> EQCSAIVPCPGGRCCSQWGYCGNTPAYCCTGCQSNCEETVCGDCPPNSGSAGDGGENGKIISRDMFDELLKRRNDLD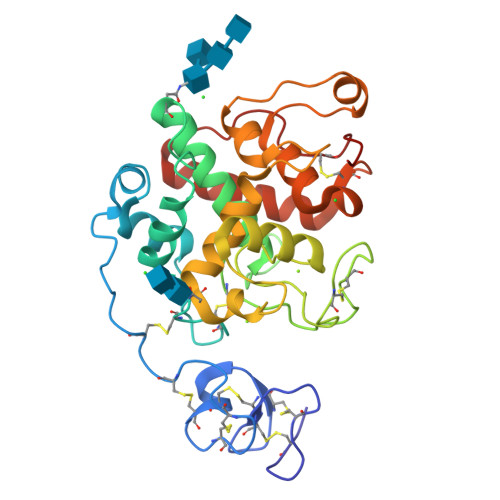CPARCFYTYNDFIQAAKAFPAFGDTGNDVIRKREIAAFFAQTSHETTGGSPGGPYQKGYCFKEEVGPGGGYCGGGYPCPDPGQYYGRGPIQLTWNYNYIFCGDDINQDLDNHPNLNSVNGVLSFKSAIWFWMTPQSPKPSCHDVMTNEWAPGGADGNAGRDPGFGLTTNIINGGLECGFGTDSRVQDRIGYFKHFCSNFGIDPGNNLDCYTQTPY>[2x]MKNQWQHQYFLSYSELVANFPSPEKVVSDYIKHKFSTTLPWFGWADPDNLYFIRFTQSRSNNKSYTGWDHLGKYAIETLTLTQAAIVNIGSR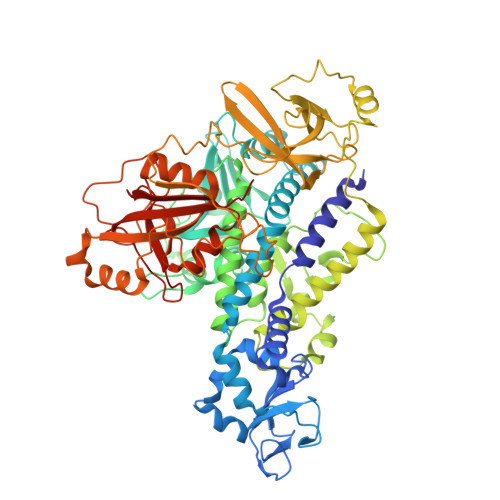FDIFDEANSTAGIYKTNNADSFDETNEAKMLPSEYLYFLRDCDFSNLYNKALSDYWAENYEKFSTLLQNYYISSAYYLYKDSAISKDEYEFSIDAIFNKKNKILRYYFDVYGYYSSDMFVAMNDNKTMLFIPGATNPFIFADNITDLRDKIKALISDKNTRELFSKHFSLYDRQDGNTYLGVNSMLEQIVSGVVDTNYIMYSNKNIRERNVFESMAFSTRERSFNDGDVIIKSNAEVQRDYALNVLQTILSLSPIFDIVLPEVSIPISLGITASSVGISFDELINGDTYEERRSAIPGLATNAVLLGISFAIPFLISKAEENKLIINNLVGSDENILNKNNLGDFLEKYNISESDIPENGSLVINLKNTNVPVRLVKLNDEEGEIVAIKGSTLSGIYYEVDTETGYEILSRRVFRTEYNEKIYWTRGGGLKGGQPFNFEGLDIPVYFIDKPYSELASSVELSFVNDDSPLLFPEMDSRLPKPTPELDIKYYSSNLSSFKEDTVILMRGTTEEEAWNIANYKTAGGSNKDLEENFIEAGPQFNLSFSEYTSSINSADTASRKHFLVIIKVQVKYISNDNVLYANHWAIPDEAPVEVLAVVDRRFIFPEPPVKP> MEEQREILEQLKKTLQMLT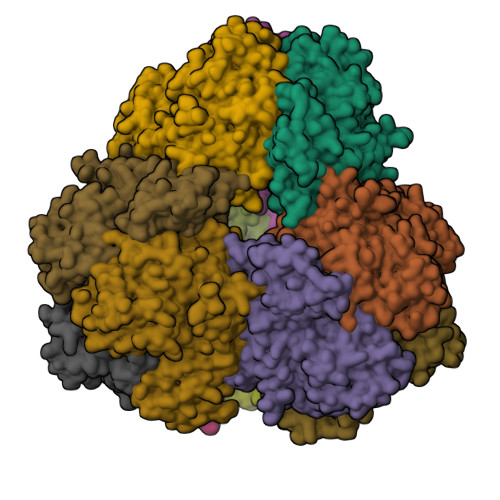VEPSKNNQIANEEKEKKENENSWCILEHNYEDIAQEFIDFIYKNPTTYHVVSFFAELLDKHNFKYLSEKSNWQDSIGEDGGKFYTIRNGTNLSAFILGKNWRAEKGVGVIGSHVDALTVKLKPVSFKDTAEGYGRIAVAPYGGTLNELWLDRDLGIGGRLLYKKKGTNEIKSALVDSTPLPVCRIPSLAPHFGKPAEGPFDKEDQTIPVIGFPTPDEEGNEPPTDDEKKSPLFGKHCIHLLRYVAKLAGVEVSELIQMDLDLFDVQKGTIGGIGKHFLFAPRLDDRLCSFAAMIALICYAKDVNTEESDLFSTVTLYDNEEIGSLTRQGAKGGLLESVVERSSSAFTKKPVDLHTVWANSIILSADVNHLYNPNFPEVYLKNHFPVPNVGITLSLDPNGHMATDVVGTALVEELARRNGDKVQYFQIKNNSRSGGTIGPSLASQTGARTIDLGIAQLSMHSIRAATGSKDVGLGVKFFNGFFKHWRSVYDEFGEL> SPGQGTQSENSCTHFPGNLPNMLRDLRDAFSRVKTFFQMKDQLDNLLLKESLLEDFKGYLGCQALSEMIQFYLEEVMPQAENQDPDIKAHVNSLGENLKTLRLRLRRCHRFLPCENKSKAVEQVKNAFNKLQEKGIYKAMSEF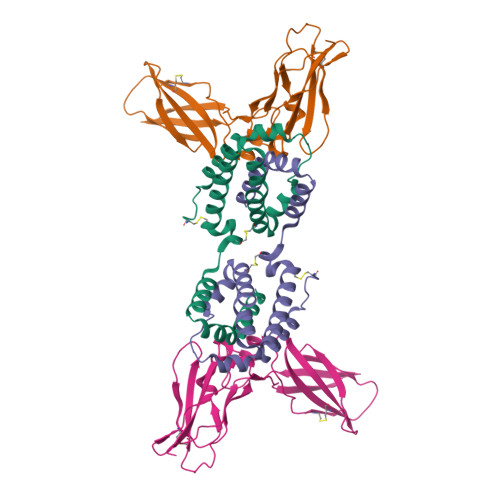DIFINYIEAYMTMKIRN;> HGTELPSPPSVWFEAEFFHHILHWTPIPQQSESTCYEVALLRYGIESWNSISQCSQTLSYDLTAVTLDLYHSNGYRARVRAVDGSRHSQWTVTNTRFSVDEVTLTVGSVNLEIHNGFILGKIQLPRPKMAPAQDTYESIFSHFREYEIAIRKVPGQFTFTHKKVKHEQFSLLTSGEVGEFCVQVKPSVASRSNKGMWSKEECISLTRQYFTVTN>[7x]NLIPTVIEQTNRGERAY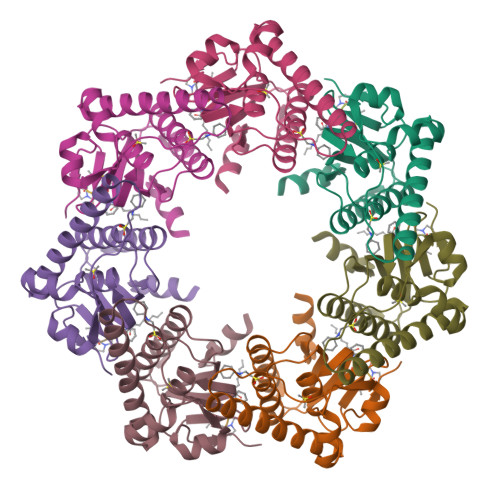DIYSRLLKDRIIMLGSAIDDNVANSIVSQLLFLAAEDPEKEISLYINSPGGSITAGMAIYDTMQFIKPKVSTICIGMAASMGAFLLAAGEKGKRYALPNSEVMIHQPLGGAQGQATEIEIAAKRILLLRDKLNKVLAERTGQPLEVIERDTDRDNFKSAEEALEYGLIDKILTHTEDKKHHH;>[7x]XFSPAAP>[4x]SVGTFSLPALPY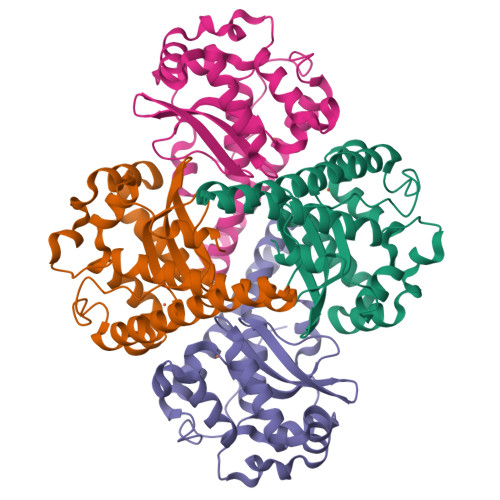AYDALEPSISAQIMELHHSKHHQTYVTNLNNALKTYSTALAANDVPSQIALQAAIKFNGGGHINHSLFWENLCPASSPDADPASAPELTAEIAKTWGSLDKFKEAMGKALLGIQGSGWGWLVKEGSGLRIVTTKDQGPVVGGEVPVFGIDMWEHAYYLQYLNGKAAYVDNIWKVINWKTAEQRFKGDREDAFKILKASL>MSTDDGRRPIRRALISVYDKTGLVDLAQGLSAAGVEIISTGSTAKTIADTGIPVTPVEQLTGFPEVLDGRVKTLHPRVHAGLLADLRKSEHAAALEQLGIEAFELVVVNLYPFSQTVESGASVDDCVEQIDIGGPAMVRAAAKNHPSAAVVTDPLGYHGVLAALRAGGFTLAERKRLASLAFQHIAEYDIAVASWMQQTLAPEHPVAAFPQWFGRSWRRVAMLRYGENPHQQAALYGDPTAWPGLAQAEQLHGKDMSYNNFTDADAAWRAAFDHEQTCVAIIKHANPCGIAISSVSVADAHRKAHECDPLSAYGGVIAANTEVSVEMAEYVSTIFTEVIVAPGYAPGALDVLARKKNIRVLVAAEPLAGGSELRPISGGLLIQQSDQLDAHGDNPANWTLATGSPADPATLTDLVFAWRACRAVKSNAIVIAADGATVGVGMGQVNRVDAARLAVERGGERVRGAV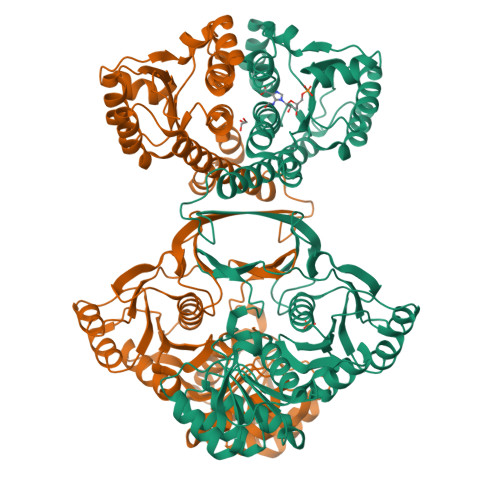AASDAFFPFPDGLETLAAAGVTAVVHPGGSVRDEEVTEAAAKAGVTLYLTGARHFAH[2x]>[3x]GAMDKENKKLLCRKCKALACYTADVRVIEECHYTVLGDAFKECFVSRPHPKPKQFSSFEKRAKI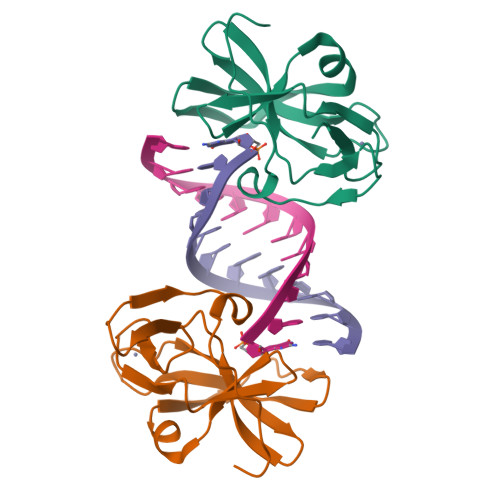FCARQNCSHDWGIHVKYKTFEIPVIKIESFVVEDIATGVQTLYSKWKDFHFEKIPFDPAEMSK> RTAKRSDVYIAGFFPYGDGVENSYTGRGVMPSVKLALGHVNEHGKILANYRLHMWWNDTQCNAAVGVKSFFDMMHSGPNKVMLFGAACTHVTDPIAKASKHWHLTQLSYADTHPMFTKDAFPNFFRVVPSENAFNAPRLALLKEFNWTRVGTVYQNEPRYSLP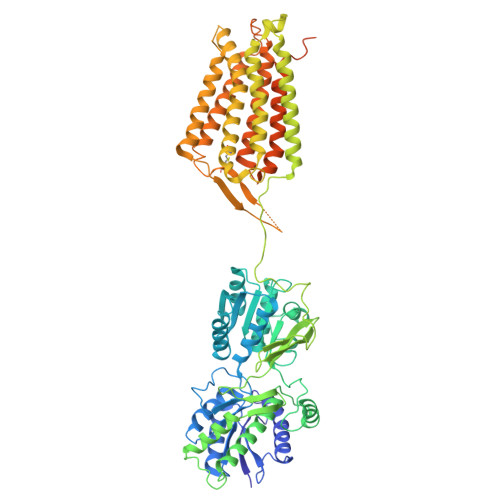HNHMVADLDAMEVEVVETQSFVNDVAESLKKLREKDVRIILGNFNEHFARKAFCEAYKLDMYGRAYQWLIMATYSTDWWNVTQDSECSVEEIATALEGAILVDLLPLSTSGDITVAGITADEYLVEYDRLRGTEYSRFHGYTYDGIWAAALAIQYVAEKREDLLTHFDYRVKDWESVFLEALRNTSFEGVTGPVRFYNNERKANILINQFQLGQMEKIGEYHSQKSHLDLSLGKPVKWVGKTPPKDRTLIYIEHSQVNPTIYIVSASASVIGVIIATVFLAFNIKYRNQRYIKMSSPHLNNLIIVGCMITYLSIIFLGLDTTLSSVAAFPYICTARAWILMAGFSLSFGAMFSKTWRVHSIFTDLKLNKKVIKDYQLFMVVGVLLAIDIAIITTWQIADPFYRETKQLEPLHHENIDDVLVIPENEYCQSEHMTIFVSIIYAYKGLLLVFGAFLAWETRHVSIPALNDSKHIGFSVYNVFITCLAGAAISLVLSDRKDLVFVLLSFFIIFCTTATLCLVFVPKLVELKRNPQGVVDKRVRATLRPMSKNGRRDSSVCELEQRLRDVKNTNCRFRKALMEKENELQALIRKLGPEARKWIDGVTC>GSHMASSAENEIEMRICDYLRRHGRSTVQDIFKELKLEKSTVN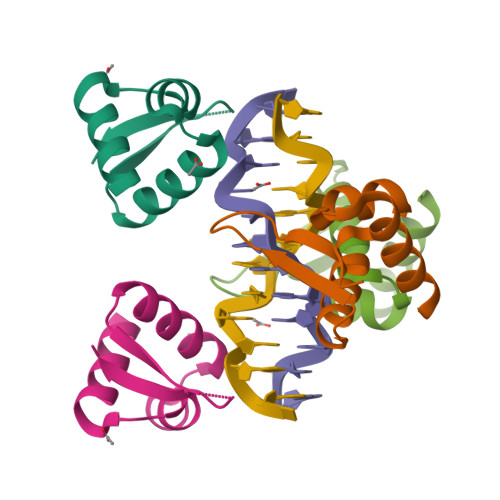RHLYSLQASKQVFKTVEDNKRPVWNLVES[2x]> MSKKQIQPVTRGRAKVPVIMQMEALECGAASLAMVLAYYKKWVPLEQVRVDCGVSRDG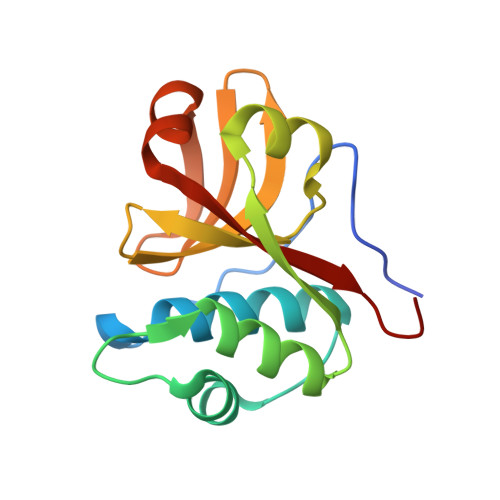SNALNVLKAARNYGLEAKGYRYEPEKLKKEGTFPCIIHWNFNHFVVLKGFKGKYAYINDPAKGDVKIPMEEFDRSFTGICLIFKPTDRF> AVAFYIP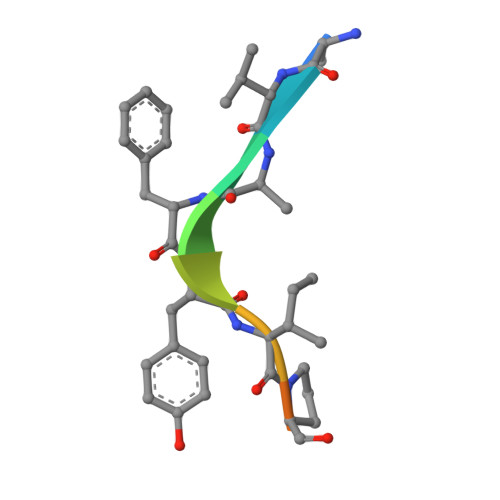DQA>[2x]MDIAKWVEHARTCYSTQLDTKIKVIGVIGKDYPDHGKGDNINCYLRENVFPVAATEDETCTIRGHFSEDDQILFLVMNGVDDVANIRKCLKSNPKSNYFDAMAESECQQIRMLHFLFISCHFIIIFEQTSRIDLELMRFLKKVNSARIQLRKKINQRLVASDLRDVSFNNRILSSAESEGRMVVPRLLIAFQRNNIRPDVNPGKKLQRELYEKLEKNLDNQFSDILKLYDLIDCGASSLCQLNETIPVVHLLNPKIVKRDIIGEMFEILMADAENTKISGNAGTLPSNNSFVKFLEDNFRSEKNEISLENVIELMNCLQCVLDGDLEEKHEKTAIQTFIKRIQNDHMEEARRLYTNAQRPGERRGADRFKDSEKPVKIRSKEEHLMRFNEATHYIDSVVGVNSREALSQLQAQCNEMWQSDMRHHHHHH;> MKESVRFLTDFGEISDAISDLLTSSPNFNVISAIGPQGAGKSTLLSMLAGNNSRQMYREYVFRPVSREANEQSRHQTIQIDIYIVNHQIFLDCQPMYSFSIMEGLPKVRGGRFDDSTAMSDTLRLTAFLLYVSHTVLVVSETHYDKVIIDTLRVAEQIRPYLAIFRPKLAIDRKTNLVFIKTKASSIDLAPTVIREREELLRLSFQDSRWLKVSQEPFKTLIVLEEIRVRREHLFEEGDEPDEAASLNEFDEQIAELREELQKNREDFTVETAAMDEKKWLDMCREVIRDKTLHKTLKEYQRAMTDGVRTHFDNGFH;>MKESVRFLTDFGEISDAISDLLTSSPNFNVISAIGPQGAGKSTLLSMLAGNNSRQMYREYVFRPVSREANEQSRHQTIQIDIYIVN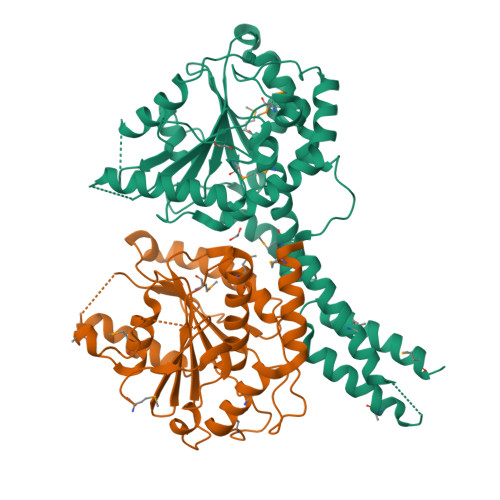HQIFLDCQPMYSFSIMEGLPKVRGGRFDDSTAMSDTLRLTAFLLYVSHTVLVVSETHYDKVIIDTLRVAEQIRPYLAIFRPKLAIDRKTNLVFIKTKASSIDLAPTVIREREELLRLSFQDSRWLKVSQEPFKTLIVLEEIRVRREHLFEEGDEPDEAASLNEFDEQIAELREELQKNREDFTVETAAMDEKKWLDMCREVIRDKTLHKTLKEYQRAMT[2x];> MDIAKWVEHARTCYSTQLDTKIKVIGVIGKDYPDHGKGDNINCYLRENVFPVAATEDETCTIRGHFSEDDQILFLVMNGVDDVANIRKCLKSNPKSNYFDAMAESECQQIRMLHFLFISCHFIIIFEQTSRIDLELMRFLKKVNSARIQLRKKINQRLVASDLRDVSFNNRILSSAESEGRMVVPRLLIAFQRNNIRPDVNPGKKLQRELYEKLEKNLDNQFSDILKLYDLIDCGASSLCQLNETIPVVHLLNPKIVKRDIIGEMFEILMADAENTKISGNAGTLPSNNSFVKFLEDNFRSEKNEISLENVIELMNCLQCVLDGDLEEKHEKTAIQTFIKRIQNDHMEEARRLYTNAQRPGERRGADRFKDSEKPVKIRSKEEHLMRFNEATHYIDSVVGVNSREALSQLQAQCNEMWQ5'-O-[(S)-{[(2S)-2-amino-3-(4-hydroxyphenyl)propanoyl]oxy}(hydroxy)phosphoryl]adenosine 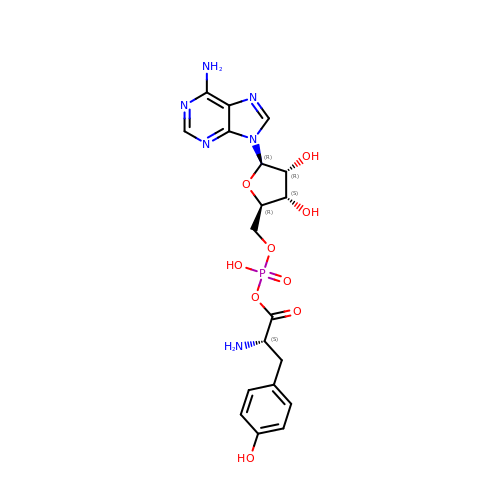| C19 H23 N6 O9 P | NFCVQVDMLQEZAK-URQYDQELSA-N>[2x]MGHHHHHHGNITLTKRQQEFLLLNGWLQLQCGHAERACILLDALLTLNPEHLAGRRCRLVALLNNNQGERAEKEAQWLISHDPLQAGNWLCLSRAQQLNGDLDKARHAYQHYLELKDHNESP;>GAMGTAQSKRSLWDFASPGYTFHGLHRAQDYRRELDTLQSLLTTSQSSELQAAAALLKCQQDDDRLLQIILNLLHKV[2x]

Several gram-negative bacteria employ type III secretion systems (T3SS) to inject effector proteins into eukaryotic host cells directly from the bacterial cytoplasm. The export gate SctV (YscV in Yersinia) binds substrate:chaperone complexes such as YscX:YscY, which are essential for formation of a functional T3SS. Here, we present structures of the YscX:YscY complex alone and bound to nonameric YscV. YscX binds its chaperone YscY at two distinct sites, resembling the heterotrimeric complex of the T3SS needle subunit with its chaperone and co-chaperone.

Our crystallization constructs contained N-terminally truncated YscX50 and full-length YscY with an N-terminal hexahistidine tag. The complex crystallized in space group P21212 with the asymmetric unit (AU) containing two heterodimers related via translational non-crystallographic symmetry. We solved the structure by molecular replacement (MR) using a model generated by AlphaFold 2. The AlphaFold 2 model correctly predicted the overall fold of the complex with YscX binding to YscY at two distinct sites connected via a short linker, resulting in YscX entwining its chaperone. Similar to other T3SCs the concave face of YscY forms an interaction site to which YscX binds via a short helix α1 (S53–A61). Moreover, this groove is largely lined by hydrophobic residues and allows for the binding of YscX’s L57, W58, F60, A61, and P63 into distinct binding pockets. A second interface is formed via the interaction of YscY’s N-terminal TPR and the two longer C-terminal α-helices (α2 and α3) of YscX. The helices of YscX are rotated by about 90° relative to YscY with the binding site containing the hydrophobic residues I3, L5, F12, L13, I31, L32, A35, and L39 for YscY as well as L80, L83, L86, L87, L95, A98, L101 and L102 for YscX. The C-terminal helix of YscX extends about 26 Å further out from where it last interacts with its chaperone, as measured from L102 to H120. In the crystal, this helix is stabilized by interacting with helix α3 of the neighboring molecule as well as the same helix from symmetry-related molecules, forming a 4-helix interface.> RSMSRPVQEMIPLKFFAVDEVSCQINQEGAPKDVVEKVLFVLNNVTLANLNNKVDELKKSLTPNYFSWFSTYLVTQRAKTEPNY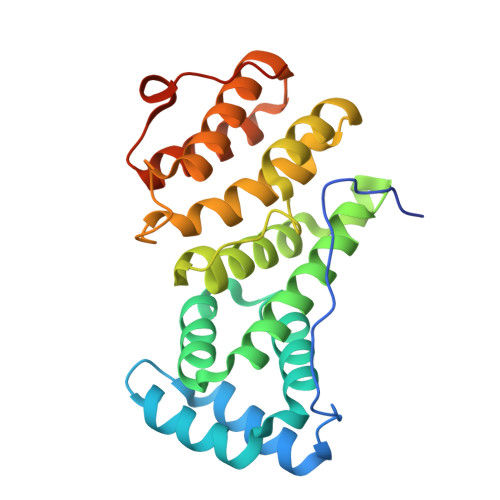HDLYSKVIVAMGSGLLHQFMVNVTLRQLFVLLSTKDEQAIDKKHLKNLASWLGCITLALNKPIKHKNIAFREMLIEAYKENRLEIVVPFVTKILQRASESKIFKPPNPWTVGILKLLIELNEKANWKLSLTFEVEVLLKSFNLTTKSLKPSNFINTPEVIETLSG2,5-dihydroxy-3-undecylcyclohexa-2,5-diene-1,4-dione | C17 H26 O4 | 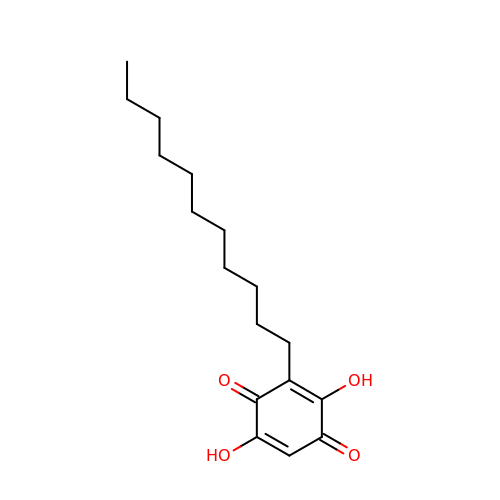IRSFLDGTOHBADP-UHFFFAOYSA-N> APTLSTDIEMIATTMSVPRQVEVTEKFKSLVTAHNGKDEEMKDVAQDMKNYMDEKYGRVWQC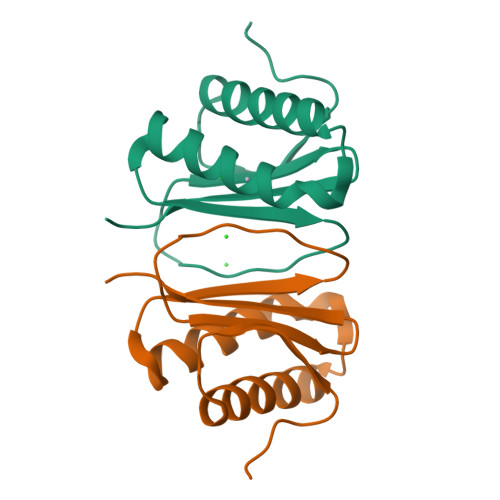VILTGSYWMHFSHEPFLSIQFRYGRHICLAWRTPRG3-(4-methoxyphenyl)benzoic 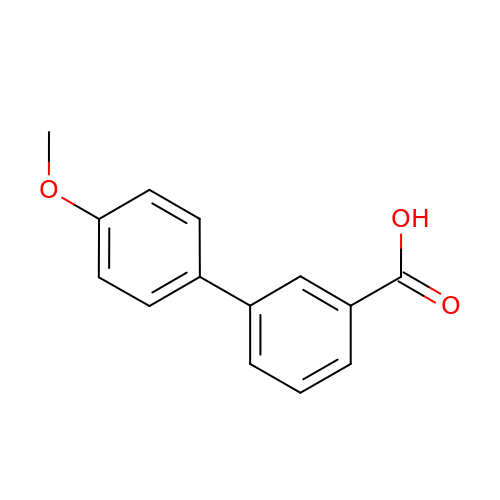acid | C14 H12 O3 | VWDMBLJBLIUXFS-UHFFFAOYSA-N1,1-Methanediyl Bismethanethiosulfonate | C3 H8 O4 S4 | 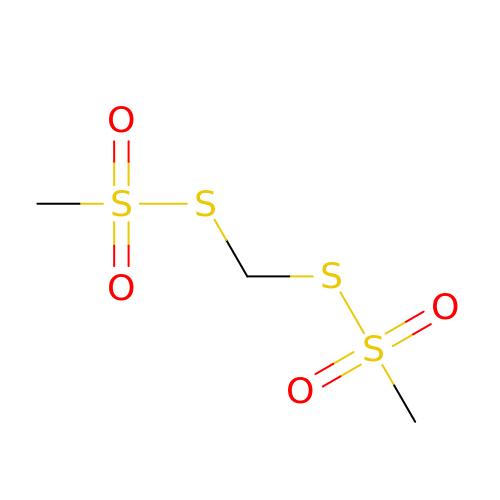SFSDVHMSSISWGL-UHFFFAOYSA-N>[4x]MASAQAVGQGERGHFVLKSGHTIPAVGL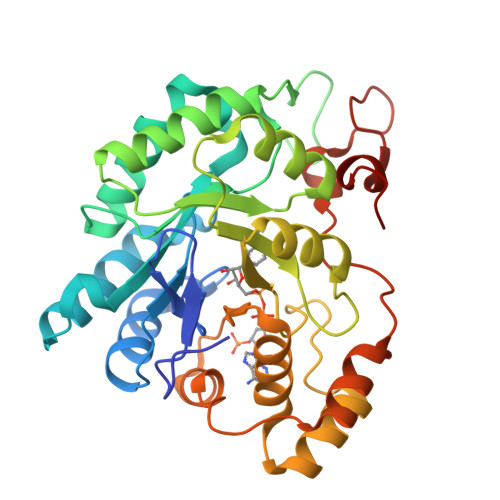GTWRAGSDTAHSVRTAIAEAGYRHVDTAAQYGVEKEVGRGLKAAMEGGINRKDLFVTSKLWCTELAPDRVRPALEKTLKDLQLDYLDLYLIHWPFRLKDGAHMPPEAGEVLELDMEGVWREMEGLVKDGLVKDIGVCNYTVAKLNRLMRSANVPPAVCQMEMHPGWKNDRIFEACKKHGIHVTAYSPLGSSEKNLAHDPLVEKVANKLDKTPGQVLLRWALQRGTSVIPKSTRDERIKENIQVFGWEIPEEDFRALCGIKDEKRVLTGEELFVNKTHGPYKSATEVWDHEDLEHHHHHH> GSTGSPPGPPEDVTIDEITDTTAQLSWRPGADNHSPITMYVVQARTPFSVGWQAVSTVPEVIDGKTFTATVVGLNPWVEYEFRVVAANLIGIGEPSRPSENRRTEEALPEVTPANVSGGGGSKSELVITWETVPEELQNGGGFGYVVAFRPFGTISWM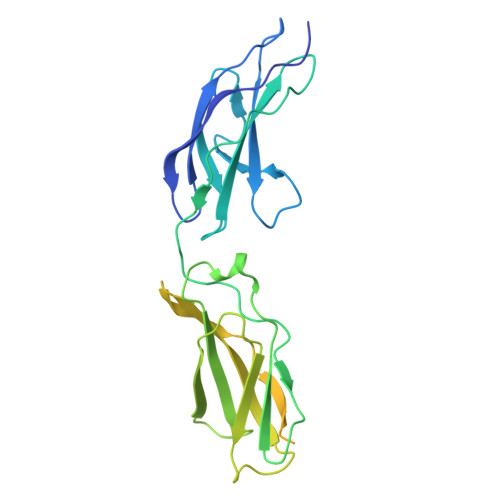QTVVASPDASRYVFRNESLPPFSPYEVKVGVYNNKGEGSFSPVTVVYSAEEEPTRAPITVLARSLSATDIEISWAPPRENQHKGRIQGYEVRCWRHDEKEENARKIRTVGNQTSAKVTNLQGNALYHLAVKAYNTAGTGPSSAMVNVTTKK>SAAYFLWPTSNLQHCAAEGRANYFGNLQKGLLPRHPGRLPKGQQANSLLDLMTIRAFHSKILRRFSLGTAVGFRIRKGDLTDIPAILVFVARKVHKKWLNPAQCLPAILEGPGGVWCDVDVVEFSYYGAPAQTPKEQMFSELVDKLCGSDECIGSGSQVASHETFGTLGAIVKRRTGNKQVGFLTNHHVAVDLDYPNQKMFHPLPPNLGPGVYLGAVERATSFITDDVWYGIYAGTNPETFVRADGAFIPFADDFDISTVTTVVRGVGDIGDVKVIDLQCPLNSLIGRQVCKVGRSSGHTTGTVMAYALEYNDEKGICFFTDILVVGENRQTFDL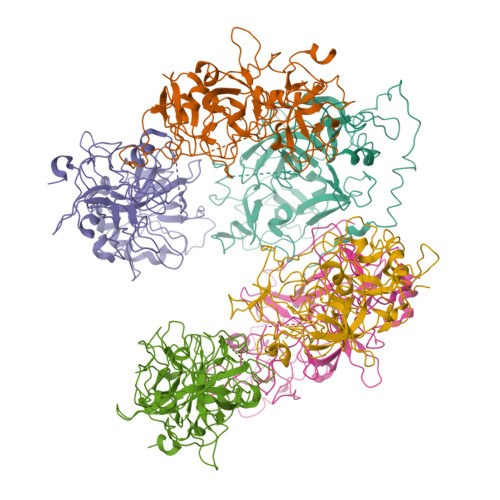EGDSGSLIILTSQDGEKPRPIGIIWGGTANRGRLKLTSDHGPENWTSGVDLGRLLDRLELDIIITNESLQDAVQ[6x]>MNQTLETGTTTVGITLKDAVIMATERRVTMENFIMHKNGKKLFQIDTYTGMTIAGLVGDAQVLVRYMKAELELYRLQRRVNMPIEAVATLLSNMLNQVKYMPYMVQLLVGGIDTAPHVFSIDAAGGSVEDIYASTGSGSPFVYGVLESQYSEKMTVDEGVDLVIRAISAAKQRDSASGGMIDVAVITRKDGYVQLPTDQIESRIRKLGLIL[14x];>AYDRAITVFSPDGRLFQVEYAREAVKKGSTALGMKFANGVLLISDKKVRSRLIEQNSIEAIQLIDDYVAAVTSGLVADARVLVDFARISAQQEKVTYGSLVNIENLVKRVADQMQQYTQYGGVRPYGVSLIFAGIDQIGPRLFDCDPAGTINEYKATAIGSGKDAVVSFLEREYKENLPEKEAVTLGIKALKSSLEEGEELKAPEIASITVGNKYRIYDQEEVKKFL[7x];>[7x]AYDRAITVFSPDGRLFQVEYALEAVKKGSTALGMKFANGVLLISDKKVRSRLIEQNSIEKIQLIDDYVAAVTSGLVADARVLVDFARIS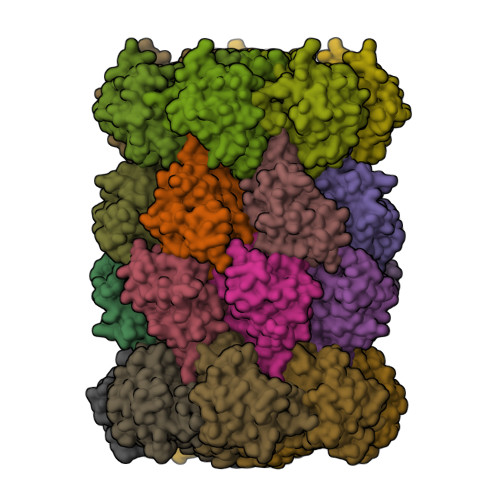AQQEKVTYGSLVNIENLVKRVADQMQQYTQYGGVRPYGVSLIFAGIDQIGPRLFDCDPAGTINEYKATAIGSGKDAVVSFLEREYKENLPEKEAVTLGIKALKSSLEEGEELKAPEIASITVGNKYRIYDQEEVKKFL>[2x]GPEASFGVLDREELEYFKQAESTLQLDAFEAPEEKFQFVTSIIEEAKGKELKLVTSQITSKLMERVILECDETQLKDIFQSFNGVFFGLSCHKYASHVLETLFVRSAALVERELLTPSFDNNEKEGPYVTMENMFLFMLNELKPHLKTMMNHQYASHVLRLLILILSSKTLPNSTKANSTLRSKKSKIARKMIDIKDNDDFNKVYQTPESFKSELRDIITTLYKGFTNGAESRSDISQSTITKFREYSVDKVASPVIQLIIQVEGIFDRDRSFWRLVFNTADEKDPKEESFLEYLLSDPVGSHFLENVIGSARLKYVERLYRLYMKDRIVKLAKRDTTGAFVVRALLEHLKEKDVKQILDAVVPELSMLLNSNMDFGTAI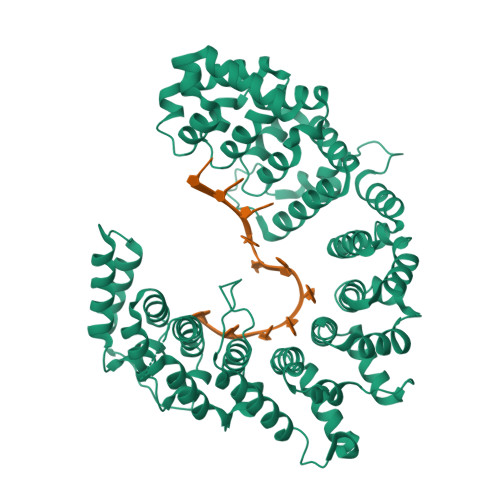INASNKQGGYLRDDVIAQLIQKYYPEKSDAKNILESCLLLSASTLGNTRDDWPTAEERRRSVFLEQLIDYDDKFLNITIDSMLALPEERLIQMCYHGVFSHVVEHVLQTTRVDIIKRKMLLNILSKESVNLACNVYGSHIMDKLWEFTAKLTLYKERIARALVLETEKVKNSIYGRQVWKNWKLELYVRKMWDWKKLIKEQEFEIFP As such, we found that a circularly permuted variant of a cage-forming enzyme, Aquifex aeolicus lumazine synthase, cpAaLS, assembles into a variety of hollow spherical and cylindrical structures in response to changes in ionic strength. Cryogenic electron microscopy revealed that these structures are composed entirely of pentameric subunits, and the dramatic cage-to-tube transformation is attributed to the moderately hindered 3-fold symmetry interaction and the imparted torsion angle of the building blocks, where both mechanisms are mediated by an α-helix domain that is untethered from the native position by circular permutation. While the wild-type protein, AaLS-wt, self-assembles into a ∼ 16 nm dodecahedral structure composed of 60 identical monomers,35 the negatively supercharged variants AaLS-neg and AaLS-13 adopt expanded 360- and 720-mer assemblies, respectively, constructed entirely from pentameric capsomers. Moreover, a circularly permuted variant of AaLS, cpAaLS(119), forms not only ∼24 nm and ∼28 nm expanded spherical cages, but also straight ∼24 nm-wide tubes of variable length. We previously designed two circularly permuted variants of AaLS and confirmed that their morphologies depend on the positions of the newly generated N- and C-termini. The native terminal amino acids were connected via an octapeptide linker using genetic fusion and new sequence termini were introduced either between residues 84 and 85 or 119 and 120, yielding cpAaLS(84) or cpAaLS(119), respectively.

The unique triple helix is not the only tubular structure formed by cpAaLS(119). In the cryo-EM micrographs, short and bent caterpillar-like objects, referred to as “twisted tubes” were also observed albeit at a very low frequency (left). However, introduction of C37S and A85C mutations into cpAaLS(119) to give cpAaLS(119, C37S, A85C) and a modified assembly protocol surreptitiously resulted in enrichment of the twisted tubular structure and allowed subsequent cryo-EM analysis (right). Since the twisted tubular assemblies were heterogeneous, we divided particle images into 3 classes and determined the structures individually. All three distinct twisted tube structures are composed of two compacted helical threads with 0-, 18-, and 28-Å gaps between them. This spring-like arrangement rationalizes the bending tendency. We also realized that one of the four pentamer interactions in the twisted tube has an acute bending angle (P0-P4 interaction). A possible disulfide bridge between two of the introduced cysteine residues at position 85 seems to support the unusual interaction mode, enhancing formation of the twisted tube.

>MTLEQAIERAGTKHGNKGWEAALSAIEMANLFKSLRGTGGSGSSMEIYEGKLTAEGLRFGIVASRFNHALVDRLVEGAIDSIVRHGGREEDITLVRVPGSWEIPVAAGELARKEDIDAVIAIGVLIRGCTPHFDYIASEVSKGLANLSLELRKPITFGVITAD[100x]> MEKSFVITDPRLPDNPIIFASDGFLELTEYSREEILGRNGRFLQGPETDQATVQKIQDAIRDQREITVQLINYTKSGKKFWNLLHLQPMRDQKGELQYFIGVQLDGEFIPNPLLALDSTRTGH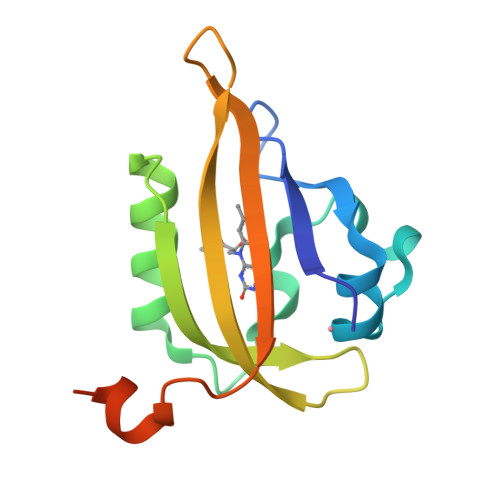HHHHH>EGRHMQEILDAILSGDAASADYAALALPESYRAVTLHKGEERMFDGLASRDKDPRKSLHLDDVPLPELGPGEALVAVMASSVNYNTVWSSIFEPVSTFGFLERYGRLSPLTARHDLPYHVLGSDLAGVVLRTGAGVNAWKPGDEVVAHCLSVELESPDGHNDTMMDPEQRIWGFETNFGGLAQLALVKTNQLLPKPKHLTWEEAASPGLVNSTAYRQLVSRNGAGLKQGDNVLIWGASGGLGSYAT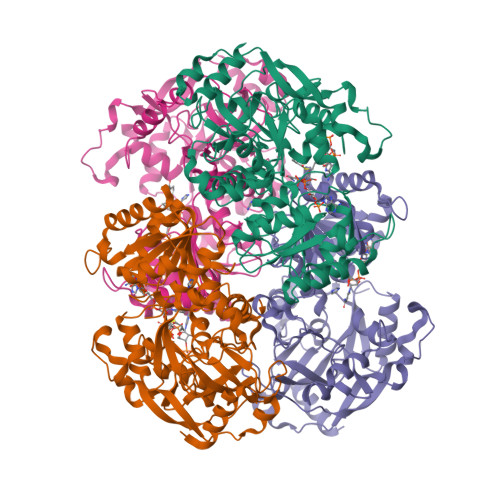QYALAGGATPICVVSSPRKADICRAMGAEAIIDRSAEGYRFWKDEHHQDPREWKRLGGKIREFTGGEDVDIVFEHPGRETFGASVYVTRKGGTIVTCASTSGYMHQYDNRYLWMSLKRIVGSHFANYREAFEANRLVAKGKIHPTLSKVYALEETGQAALDVHHNKHQGKVGVLCLAPREGLGVTDPELRSKHLTKINAFRNV[4x]>[2x]SSVLASCPKKPVSSYLRFSKEQLPIFKAQNPDAKTTELIRRIAQRWRELPDSKKKIYQDAYRAEWQVYKEEISRF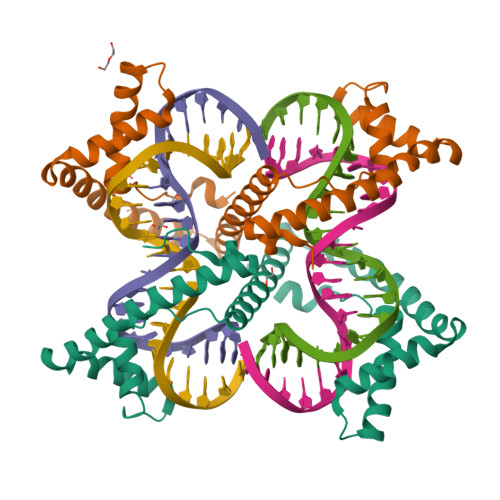KEQLTPSQIMSLEKEIMDKHLKRKAMTKKKELTLLGKPKRPRSAYNVYVAERFQEAKGDSPQEKLKTVKENWKNLSDSEKELYIQHAKEDETRYHNEMKSWEEQMIEVGRKDLLRRTIKKQRKYGAEEC> GHMGITAIALYDYQAAGDDEISFDPDDIITNIEMI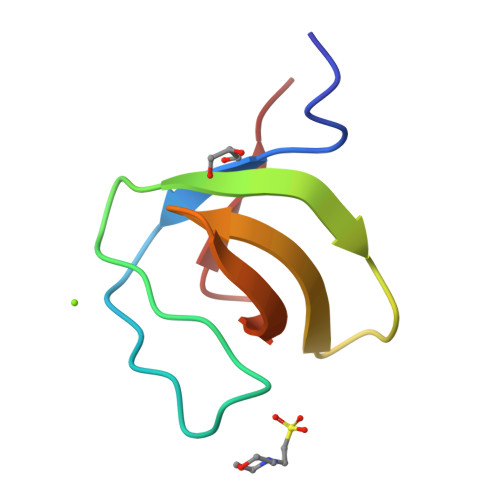DDGWWRGVCKGRYGLFPANYVELRQ> DQENMLKISGYPGMLN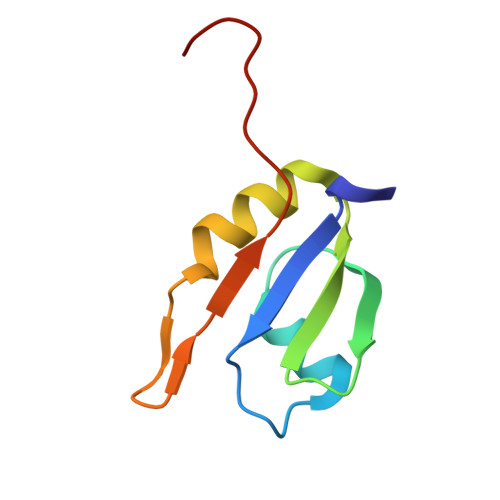TFGIAQLLTPYRVNGITITGAQSAVVALENKFQVYQAVQDFNGKKLDRNHKLQVSSLVVSSPAVPLE>GSAEVLNEDFENGIPASWKTIDADGDGNNWTTTPPPGGSSFAGHNSAICVSSASY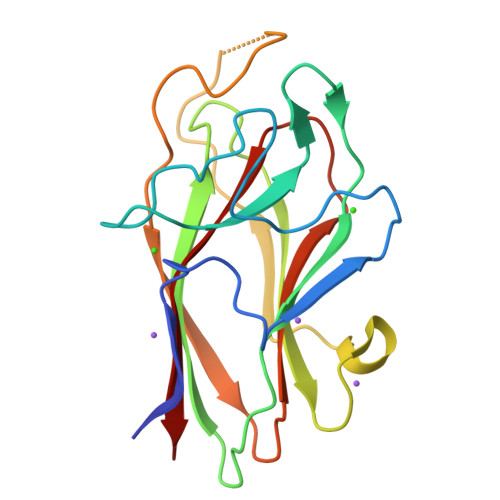INFEGPQNPDNYLVTPELSLPGGGTLTFWVCAQDANYASEHYAVYASSTGNDASNFANALLEEVLTAKTVVTAPEAIRGTRAQGTWYQKTVQLPAGTKYVAFRHFGCTDFFWINLDDVVITSG[4x]>GNPIVVVHGGGAGPISKDRKERVHQGMVRAATVGYGILREGGSAVDAVEGAVVALEDDPEFNAGCGSVLNTNGEVEMDASIMDGKDLSAGAVSAVQCIANPIKLARLVMEKTPHCFLTDQGAAQFAAAMGVPEIPGEKLVTERNKKRLEKEKHEKGAQKTDCQKNLGHHHHHHMTVGAVALDCKGNVAYATSTGGIVNKMVGRV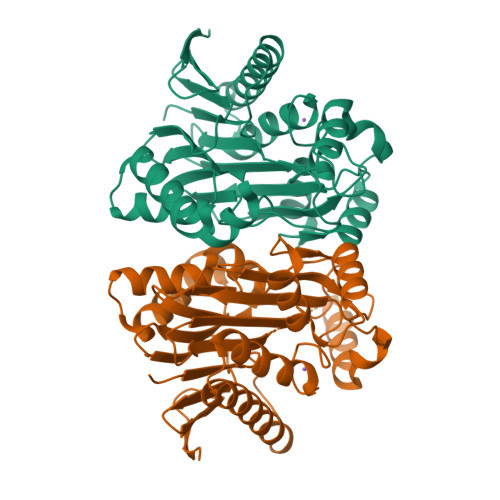GDSPCLGAGGYADNDIGAVSTTGHGESILKVNLARLTLFHIEQGKTVEEAADLSLGYMKSRVKGLGGLIVVSKTGDWVAKWTSTSMPWAAAKDGKLHFGIDPDDTTITDLPGAGSGAGSGAGG[2x]>MKVEEILEKALELVIPDEEEVRKGREAEEELRRRLDELGVEYVFVGSYARNTWLKGSLEIDVFLLFPEEFSKEELRERGLEIGKAVLDSYEIRYAEHPYVHGVVKGVEVDVVPCYKLKEPKNIKSAVDRTPFHHKWLEGRIKGKENEVRLLKGFLKANGIYGAEYKVRGFSGYLCELLIVFYGSFLETVKNARRWTRRTVIDVAKGEVRKGEEFFVVDPVDEKRNVAANLSLDNLARFVHLCREFMEAPSLGFFKPKHPLEIEPERLRKIVEERGTAVFAVKFRKPDIVDDNLYPQLERASRKIFEFLERENFMPLRSAFKAS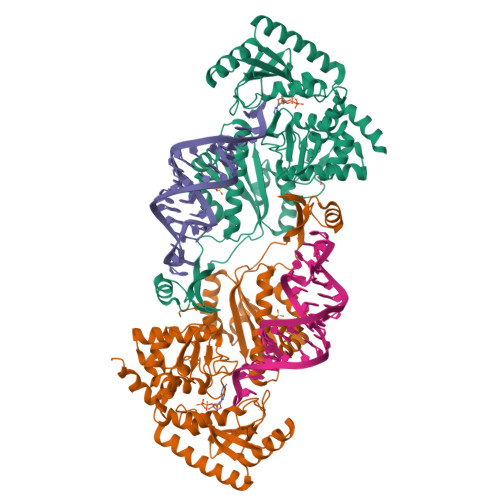EEFCYLLFECQIKEISRVFRRMGPQFEDERNVKKFLSRNRAFRPFIENGRWWAFEMRKFTTPEEGVRSYASTHWHTLGKNVGESIREYFEIISGEKLFKEPVTAELCEMMGVKDCCCM[2x]> MRVTVYGFGSLNYYSNKLNVPEKLGGEPPYGGSAMAVEFAKAGHDVTLSDPNIDKVPDEIRKKVEDAGVKLTTDDIEAAKEAEVAILFTPFRGGVTFKIAETILPYLVENAVICTTCTMSILVLNSYLQNAIFLEGREDIGFSTMHPAAIPGTPQHKHYLIATNELLRKPIVTEEQIEKLKKLATDTGKEAYLLPAELVSPVGDMGIVTTAIAFAGAIEYYKVSRDILKTKRSMTEFQIAQSLQVISSLVTKYGLEGLIKLLNVDAMKASLQS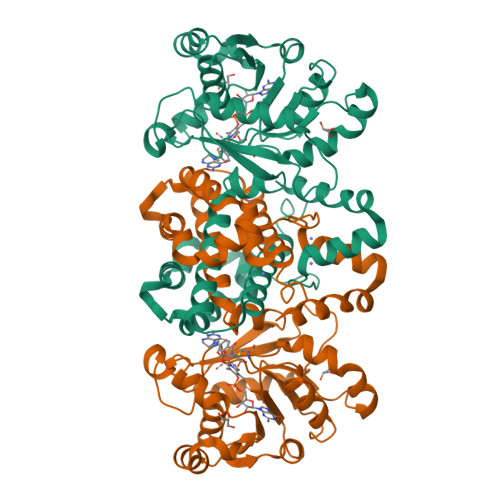MILDKNEQPLTVTASKLLEKIEETIPELIKEAENFSPSEPTYTSAPSPMLVEHMEDLVGDDVLKGILRESWKKFYENVSERNKEKLAAALEHHHHHH3-hydroxypropyl 2-acetamido-2,4-dideoxy-alpha-L-threo-hex-4-enopyranosiduronic acid 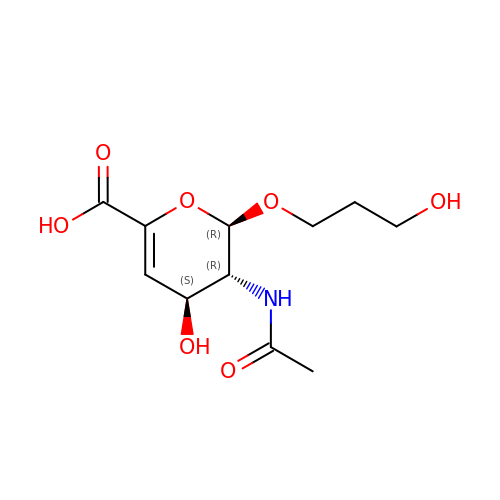| C11 H17 N O7 | MLEYNFMNPJIWGP-JVUFJMBOSA-N>[4x]MSEIGTGFPFDPHYVEVLGSRMHYVDVGPRDGTPVLFLHGNPTSSYLWRNIIPHVAPSHRCIAPDLIGMGKSDKPDLDYRFDDHVRYLDAFIEALGLEEVVLVIHDWGSALGFHWAKRNPERVKGIAFMEFIRPIPTWDEWPEFARELFQA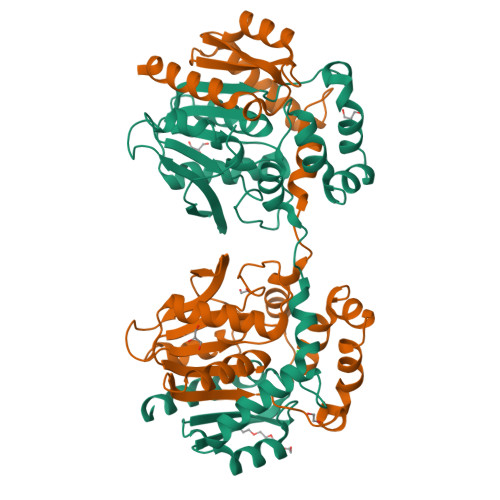FRTPDVGRELIIDQNAFIEGILPKFVVRPLTEVEMDHYREPFLKPVWREPLWRFPNELPIAGEPANIWALVEAYMNWLHQSPVPKLLFWGTPGVLIPPAEAARLAESLPNLKTVFIGPGLHYLQEDNPDLIGSEIARWLPALHHHHHH> AVNGTSQFTCFYNSRANISCVWSQDGALQDTSCQVHAWPDRRRWNQTCELLPVSQASWACNLILGAPDSQKLTTVDIVTLRVLCREGVRWRVMAIQDFKPFENLRLMAPISLQVVHVETHRCNISWEISQASHYFERHLEFEARTLSPGHTWEEAPLLTLKQKQEWICLETLTPDTQYEFQVRVKPLQGEFTTWSPWSQPLAFRTKPAALGKDTGAQDKTHTCPPCPAPELLG;> LNTTILTPNGNEDTTADFFLTTMPTDSLSVSTLPLPEVQCFVFNVEYMNCTWNSSSEPQPTNLTLHYWYKNSDNDKVQKCSHYLFSEEITSGCQLQKKEIHLYQTFVVQLQDPREP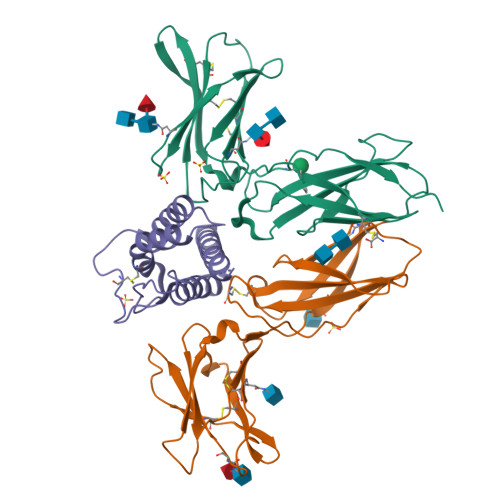RRQATQMLKLQNLVIPWAPENLTLHKLSESQLELNWNNRFLNHCLEHLVQYRTDWDHSWTEQSVDYRHKFSLPSVDGQKRYTFRVRSRFNPLCGSAQHWSEWSHPIHWGSNTSKENPFLFALEAGAQDKTHTCPPCPAPELLG;> MGWSCIILFLVATATGVHSAPASSSTKKTQLQLEHLLLDLQMILNGINNYKNPKLTRMLTAKFAMPKKATELKHLQCLEEELKPLEEVLNGAQSKNFHLRPRDLISNINVIVLELKGSETTFMCEYADETATIVEFLNRWITFAQSIISTLTVDHHHHHH> MKVGQDKVVTIRYTLQVEGEVLDQGELSYLHGHRNLIPGLEEA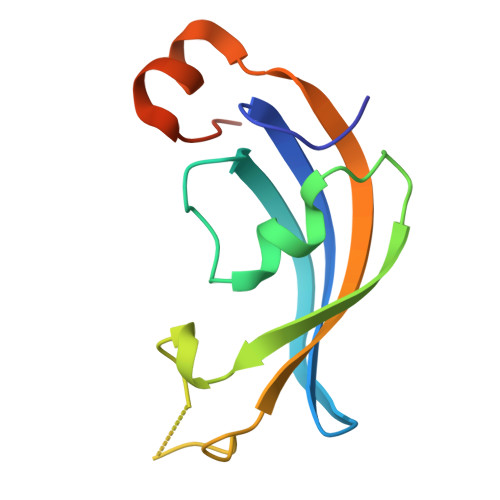LEGREEGEAFQAHVPAEKAYGATGHPGIIPPHATLDFQVEVVKVREATPEELLHGHAHPSGHHHHHH>MMSTTLFKDFTFEAAHRLPHVPEGHKCGRLHGHSFMVRLEITGEVDPHTGWIIDFAELKAAFKPTYERLDHHYLNDIPGLENPTSEVLAKWIWDQVK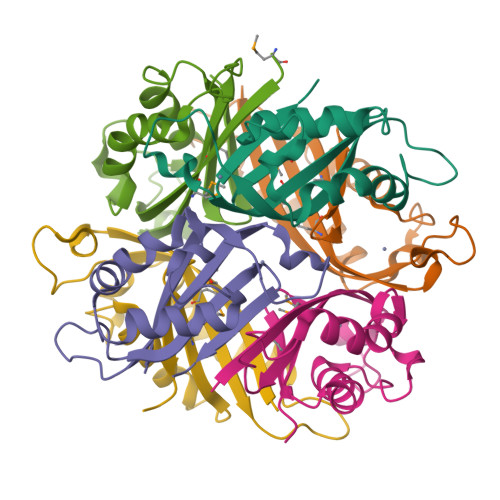PVVPLLSAVMVKETCTAGCIYRGE[6x]> ANTSSAYNSVYDFLRYHDRGDGLTVNGKTSYSIDQAAAQITRENVSWNGTNVFGKSANLTFKFLQSVSSIPSGDTGFVKFNAEQIEQAKLSLQSWSDVANLTFTEVTGNKSANITFGNYTRDASGNLDYGTQAYAYYPGNYQGAGSSWYNYNQSNIRNPGSEEYGRQTFTHEIGHALGLAHPGEYNAGEGDPSYNDAV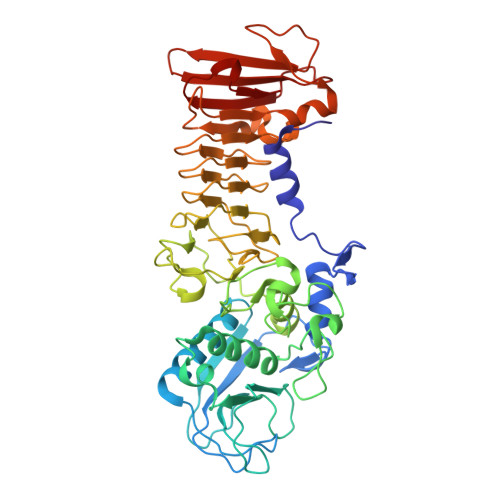YAEDSYQFSIHSYWGENETGADYNGHYGGAPMIDDIAAIQRLYGANMTTRTGDSVYGFNSNTDRDFYTATDSSKALIFSVWDAGGTDTFDFSGYSNNQRINLNEGSFSDVGGLKGNVSIAHGVTIENAIGGSGNDILVGNSADNILQGGAGNDVLYGGAGADTLYGGAGRDTFVYGSGQDSTVAAYDWIADFQKGIDKIDLSAFRNEGQLSFVQDQFTGKGQEVMLQWDAANSITNLWLHEAGHSSVDFLVRIVGQAAQSDIIV> MINTMTLDNGVRIITEKMSTVRSVSIGIWVGTGSRYESAEENGISHFLEHMFFKGTNTRSAQEIAEFFDSIGGQVNAFTSKEYTCYYAKVLDDHAGQAIDTLSDMFFHSTFQKEELEKERKVVFEEIKMVDDTPDDIVHDLLSSATYGKHSLGYPILGTVE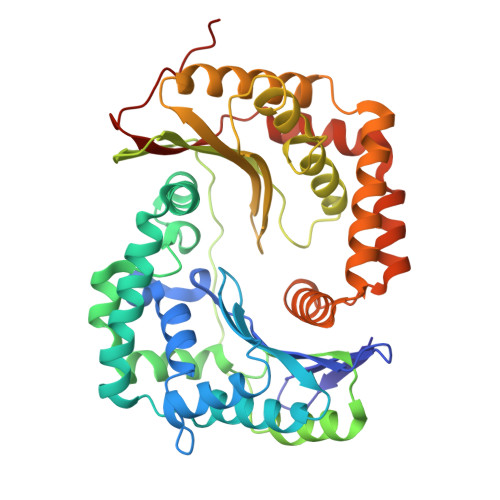TLNSFNEGMLRHYMDRFYTGDYVVISVAGNVHDELIDKIKETFSQVKPTTYNYQGEKPMFLPNRIVRKKETEQAHLCLGYPGLPIGDKDVYALVLLNNVLGGSMSSRLFQDIREKRGLCYSVFSYHSSFRDSGMLTIYAGTGHDQLDDLVYSIQETTSALAEKGLTEKELENGKEQLKGSLMLSLESTNSRMSRNGKNELLLKKHRSLDEMIEQINAVQKQDVSRLAKILLSASPSISLINANGELPKALIHLEHHHHHH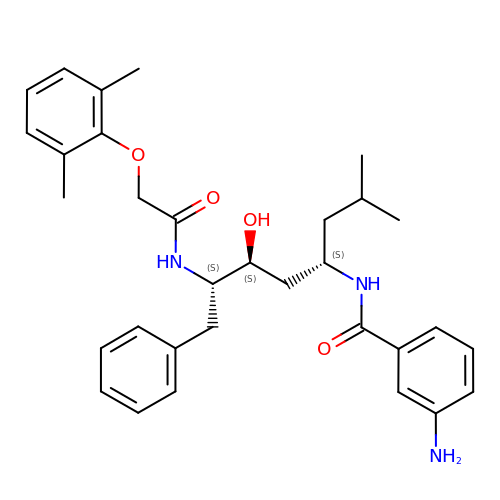4-AMINO-N-{4-[2-(2,6-DIMETHYL-PHENOXY)-ACETYLAMINO]-3-HYDROXY-1-ISOBUTYL-5-PHENYL-PENTYL}-BENZAMIDE | C32 H41 N3 O4 | WQUBEIMCFHCJCO-AWCRTANDSA-N> ELICIVQRVNESFSLHSGFGGNVYSMKTEPMTGFTNVTKGASVINQKDWIGFGDSRTDLTNDQFPASSDVPLAVAKKFRSLSGASLMLSAFGPPGKVDYLYQGCGKEKVFYEGVNWSPEAGIDCFGSNWTQTKKDFYSRIYEAARSSTCMTLVNSLDTKISSTTATAGTASSCSSSWMKSPLWYAESSVNPGAKPQVCGTEQSATFTLPTSFGIYKCNKHVVQLCYFVYENKAKFNTFGCGDYYQNYYDGNGNLIGGMDN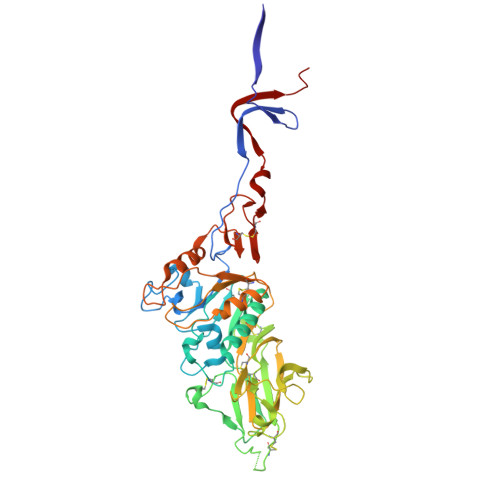RVAAYRGIANAGVKIECPSKILNPGTYSIKSTPRFLLVPKRSYCFDTDGGYPIQVVQSEWSASRRSDNATEEACLQTEGCIFIKKTTPYVGEADDNHGDIEMRQLLSGLGNNDTVCVSQSGYTKGETPFVKDYLSPPKYGRCQLKTDSGRIPTLPSGLIIPQAGTDS> MAREVKLTKAGYERLMQQLERERERLQEATK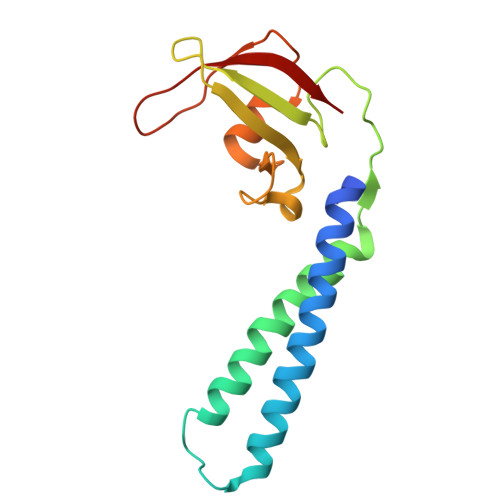ILQELMESSDDYDDSGLEAAKQEKARIEARIDSLEDILSRAVILEEGSGEVIGLGSVVELEDPLSGERLSVQVVSPAEANVLDTPMKISDASPMGKALLGHRVGDVLSLDTPKGRREFRVVAIHG>[4x]HVGCVVSWKNKELKCGSGIFITDNVHTWTEQYKFQPESPSKLASAIQKAHEEGICGIRSVTRLENLMWKQITPELNHILTENEVKLTIMTGDIKGIMQAGKRSLRPQPTELKYSWKAWGKAKMLSTELHNH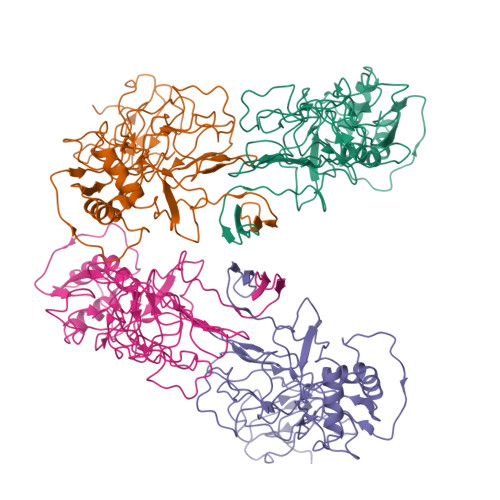TFLIDGPETAECPNTNRAWNSLEVEDYGFGVFTTNIWLKLKERQDVFCDSKLMSAAIKDNRAVHADMGYWIESALNDTWKIEKASFIEVKSCHWPKSHTLWSNGVLESEMIIPKNFAGPVSQHNYRPGYHTQTAGPWHLGRLEMDFDFCEGTTVVVTEDCGNRGPSLRTTTASGKLITEWCCRSCTLPPLRYRGEDGCWYGMEIRPLKEK> GSHMAKVQVNNVVVLDNPSPFYNPFQFEITFECIEDL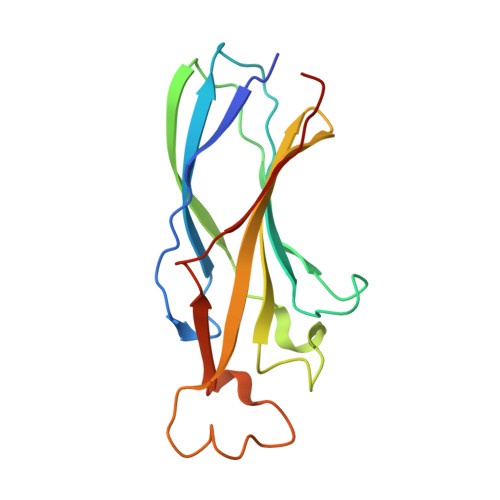SEDLEWKIIYVGSAESEEYDQVLDSVLVGPVPAGRHMFVFQADAPNPGLIPDADAVGVTVVLITCTYRGQEFIRVGYYVNNEYTETELRENPPVKPDFSKLQRNILASNPRVTRFHINWED5-(propan-2-yl)-2-thioxodihydropyrimidine-4,6(1H,5H)-dione | C7 H10 N2 O2 S | 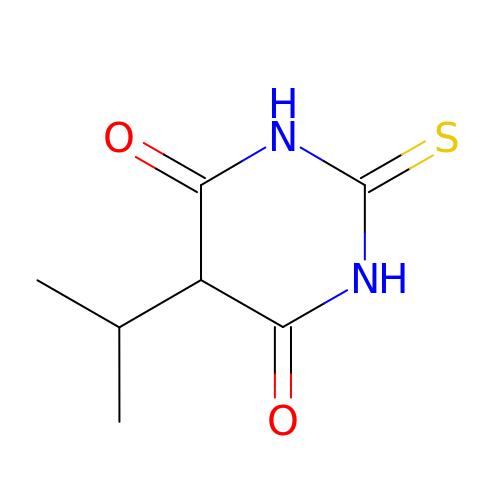QWVRNSPNBZGMRZ-UHFFFAOYSA-N5-[3-chloranyl-2-fluoranyl-6-(1,2,3,4-tetrazol-1-yl)phenyl]-2-[(1~{R})-2-cyclopropyl-1-[4-(3-methylimidazol-4-yl)pyrazol-1-yl]ethyl]-1-oxidanyl-pyridine | C24 H21 Cl F N9 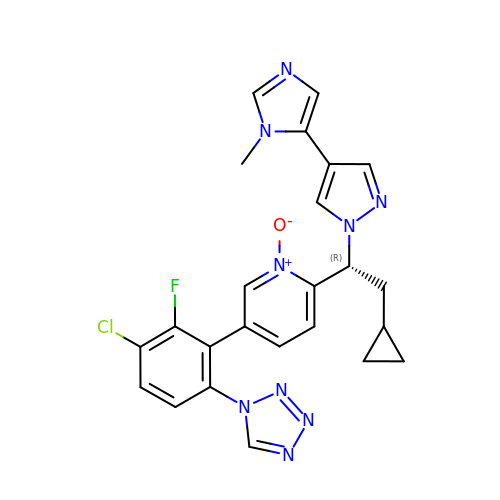O | IQYPMNRUPQZQQR-OAQYLSRUSA-N>[2x]GPMVTGGGAAPPGTVTEPLPSVIVLSAGRKMAAAAAAASGPGCSSAAGAGAAGVSEWLVLRDGCMHCDADGLHSLSYHPALNAILAVTSRGTIKVIDGTSGATLQASALSAKPGGQVKCQYISAVDKVIFVDDYAVGCRKDLNGILLLDTALQTPVSKQDDVVQLELPVTEAQQLLSACLEKVDISSTEGYDLFITQLKDGLKNTSHETAANHKVAKWATVTFHLPHHVLKSIASAIVNELKKINQNVAALPVASSVMDRLSYLLPSARPELGVGPGRSVDRSLMYSEANRRETFTSWPHVGYRWAQPDPMAQAGFYHQPASSGDDRAMCFTCSVCLVCWEPTDEPWSEHERHSPNCPFVKGEHTQNVPLSVTLATSPAQFPCTDGTDRISCFGSGSCPHFLAAATKRGKICIWDVSKLMKVHLKFEINAYDPAIVQQLILSGDPSSGVDSRRPTLAWLEDSSSCSDIPKLEGDSDDLLEDSDSEEHSRSDSVTGHTSQKEAMEVSLDITALSILQQPEKLQWEIVANVLEDTVKDLEELGANPCLTNSKSEKTKEKHQEQHNIPFPCLLAGGLLTYKSPATSPISSNSHRSLDGLSRTQGESISEQGSTDNESCTNSELNSPLVRRTLPVLLLYSIKESDEKAGKIFSQMNNIMSKSLHDDGFTVPQIIEMELDSQEQLLLQDPPVTYIQQFADAAANLTSPDSEKWNSVFPKPGTLVQCLRLPKFAEEENLCIDSITPCADGIHLLVGLRTCPVESLSAINQVEALNNLNKLNSALCNRRKGELESNLAVVNGANISVIQHESPADVQTPLIIQPEQRNVSGGYLVLYKMNYATRIVTLEEEPIKIQHIKDPQDTITSLILLPPDILDNREDDCEEPIEDMQLTSKNGFEREKTSDISTLGHLVITTQGGYVKILDLSNFEILAKVEPPKKEGTEEQDTFVSVIYCSGTDRLCACTKGGELHFLQIGGTCDDIDEADILVDGSLSKGIEPSSEGSKPLSNPSSPGISGVDLLVDQPFTLEILTSLVELTRFETLTPRFSATVPPCWVEVQQEQQQRRHPQHLHQQHHGDAAQHTRTWKLQTDSNSWDEHVFELVLPKACMVGHVDFKFVLNSNITNIPQIQVTLLKNKAPGLGKVNALNIEVEQNGKPSLVDLNEEMQHMDVEESQCLRLCPFLEDHKEDILCGPVWLASGLDLSGHAGMLTLTSPKLVKGMAGGKYRSFLIHVKAVNERGTEEICNGGMRPVVRLPSLKHQSNKGYSLASLLAKVAAGKEKSSNVKNENTSGTRKSENLRGCDLLQEVSVTIRRFKKTSISKERVQRCAMLQFSEFHEKLLNTLCRKTDDGQITEHAQSLVLDTLCWLAGVHSNGPGSSKEGNENLLSKTRKFLSDIVRVCFFEAGRSIAHKCARFLALCISNGKCDPCQPAFGPVLLKALLDNMSFLPAATTGGSVYWYFVLLNYVKDEDLAGCSTACASLLTAVSRQLQDRLTPMEALLQTRYGLYSSPFDPVLFDLEMSGSSCKNVYNSSIGVQSDEIDLSDVLSGNGKVSSCTAAEGSFTSLTGLLEVEPLHFTCVSTSDGTRIERDDAMSSFGVTPAVGGLSSGTVGEASTALSSAAQVALQSLSHAMASAEQQLQVLQEKQQQLLKLQQQKAKLEAKLHQTTAAAAAAASAVGPVHNSVPSNPVAAPGFFIHPSDVIPPTPKTTPLFMTPPLTPPNEAVSVVINAELAQLFPGSVIDPPAVNLAAHNKNSNKSRMNPLGSGLALAISHASHFLQPPPHQSIIIERMHSGARRFVTLDFGRPILLTDVLIPTCGDLASLSIDIWTLGEEVDGRRLVVATDISTHSLILHDLIPPPVCRFMKITVIGRYGSTNARAKIPLGFYYGHTYILPWESELKLMHDPLKGEGESANQPEIDQHLAMMVALQEDIQCRYNLACHRLETLLQSIDLPPLNSANNAQYFLRKPDKAVEEDSRVFSAYQDCIQLQLQLNLAHNAVQRLKVALGASRKMLSETSNPEDLIQTSSTEQLRTIIRYLLDTLLSLLHASNGHSVPAVLQSTFHAQACEELFKHLCISGTPKIRLHTGLLLVQLCGGERWWGQFLSNVLQELYNSEQLLIFPQDRVFMLLSCIGQRSLSNSGVLESLLNLLDNLLSPLQPQLPMHRRTEGVLDIPMISWVVMLVSRLLDYVATVEDEAAAAKKPLNGNQWSFINNNLHTQSLNRSSKGSSSLDRLYSRKIRKQLVHHKQQLNLLKAKQKALVEQMEKEKIQSNKGSSYKLLVEQAKLKQATSKHFKDLIRLRRTAEWSRSNLDTEVTTAKESPEIEPLPFTLAHERCISVVQKLVLFLLSMDFTCHADLLLFVCKVLARIANATRPTIHLCEIVNEPQLERLLLLLVGTDFNRGDISWGGAWAQYSLTCMLQDILAGELLAPVAAEAMEEGTVGDDVGATAGDSDDSLQQSSVQLLETIDEPLTHDITGAPPLSSLEKDKEIDLELLQDLMEVDIDPLDIDLEKDPLAAKVFKPISSTWYDYWGADYGTYNYNPYIGGLGIPVAKPPANTEKNGSQTVSVSVSQALDARLEVGLEQQAELMLKMMSTLEADSILQALTNTSPTLSQSPTGTDDSLLGGLQAANQTSQLIIQLSSVPMLNVCFNKLFSMLQVHHVQLESLLQLWLTLSLNSSSTGNKENGADIFLYNANRIPVISLNQASITSFLTVLAWYPNTLLRTWCLVLHSLTLMTNMQLNSGSSSAIGTQESTAHLLVSDPNLIHVLVKFLSGTSPHGTNQHSPQVGPTATQAMQEFLTRLQVHLSSTCPQIFSEFLLKLIHILSTERGAFQTGQGPLDAQVKLLEFTLEQNFEVVSVSTISAVIESVTFLVHHYITCSDKVMSRSGSDSSVGARACFGGLFANLIRPGDAKAVCGEMTRDQLMFDLLKLVNILVQLPLSGNREYSARVSVTTNTTDSVSDEEKVSGGKDGNGSSTSVQGSPAYVADLVLANQQIMSQILSALGLCNSSAMAMIIGASGLHLTKHENFHGGLDAISVGDGLFTILTTLSKKASTVHMMLQPILTYMACGYMGRQGSLATCQLSEPLLWFILRVLDTSDALKAFHDMGGVQLICNNMVTSTRAIVNTARSMVSTIMKFLDSGPNKAVDSTLKTRILASEPDNAEGIHNFAPLGTITSSSPTAQPAEVLLQATPPHRRARSAAWSYIFLPEEAWCDLTIHLPAAVLLKEIHIQPHLASLATCPSSVSVEVSADGVNMLPLSTPVVTSGLTYIKIQLVKAEVASAVCLRLHRPRDASTLGLSQIKLLGLTAFGTTSSATVNNPFLPSEDQVSKTSIGWLRLLHHCLTHISDLEGMMASAAAPTANLLQTCAALLMSPYCGMHSPNIEVVLVKIGLQSTRIGLKLIDILLRNCAASGSDPTDLNSPLLFGRLNGLSSDSTIDILYQLGTTQDPGTKDRIQALLKWVSDSARVAAMKRSGRMNYMCPNSSTVEYGLLMPSPSHLHCVAAILWHSYELLVEYDLPALLDQELFELLFNWSMSLPCNMVLKKAVDSLLCSMCHVHPNYFSLLMGWMGITPPPVQCHHRLSMTDDSKKQDLSSSLTDDSKNAQAPLALTESHLATLASSSQSPEAIKQLLDSGLPSLLVRSLASFCFSHISSSESIAQSIDISQDKLRRHHVPQQCNKMPITADLVAPILRFLTEVGNSHIM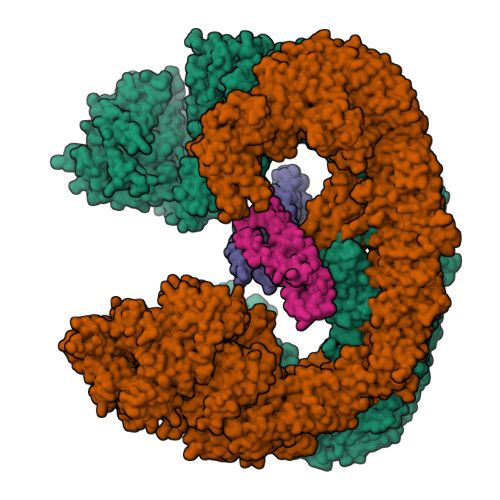KDWLGGSEVNPLWTALLFLLCHSGSTSGSHNLGAQQTSARSASLSSAATTGLTTQQRTAIENATVAFFLQCISCHPNNQKLMAQVLCELFQTSPQRGNLPTSGNISGFIRRLFLQLMLEDEKVTMFLQSPCPLYKGRINATSHVIQHPMYGAGHKFRTLHLPVSTTLSDVLDRVSDTPSITAKLISEQKDDKEKKNHEEKEKVKAENGFQDNYSVVVASGLKSQSKRAVSATPPRPPSRRGRTIPDKIGSTSGAEAANKIITVPVFHLFHKLLAGQPLPAEMTLAQLLTLLYDRKLPQGYRSIDLTVKLGSRVITDPSLSKTDSYKRLHPEKDHGDLLASCPEDEALTPGDECMDGILDESLLETCPIQSPLQVFAGMGGLALIAERLPMLYPEVIQQVSAPVVTSTTQEKPKDSDQFEWVTIEQSGELVYEAPETVAAEPPPIKSAVQTMSPIPAHSLAAFGLFLRLPGYAEVLLKERKHAQCLLRLVLGVTDDGEGSHILQSPSANVLPTLPFHVLRSLFSTTPLTTDDGVLLRRMALEIGALHLILVCLSALSHHSPRVPNSSVNQTEPQVSSSHNPTSTEEQQLYWAKGTGFGTGSTASGWDVEQALTKQRLEEEHVTCLLQVLASYINPVSSAVNGEAQSSHETRGQNSNALPSVLLELLSQSCLIPAMSSYLRNDSVLDMARHVPLYRALLELLRAIASCAAMVPLLLPLSTENGEEEEEQSECQTSVGTLLAKMKTCVDTYTNRLRSKRENVKTGVKPDASDQEPEGLTLLVPDIQKTAEIVYAATTSLRQANQEKKLGEYSKKAAMKPKPLSVLKSLEEKYVAVMKKLQFDTFEMVSEDEDGKLGFKVNYHYMSQVKNANDANSAARARRLAQEAVTLSTSLPLSSSSSVFVRCDEERLDIMKVLITGPADTPYANGCFEFDVYFPQDYPSSPPLVNLETTGGHSVRFNPNLYNDGKVCLSILNTWHGRPEEKWNPQTSSFLQVLVSVQSLILVAEPYFNEPGYERSRGTPSGTQSSREYDGNIRQATVKWAMLEQIRNPSPCFKEVIHKHFYLKRVEIMAQCEEWIADIQQYSSDKRVGRTMSHHAAALKRHTAQLREELLKLPCPEGLDPDTDDAPEVCRATTGAEETLMHDQVKPSSSKELPSDFQL;>AVPIAQKSEPHSLSSEALMRRAVSLVTDSTSTFLSQTTYALIEAITEYTKAVYTLTSLYRQYTSLLGKMNSEEEDEVWQVIIGARAEMTSKHQEYLKLETTWMTAVGLSEMAAEAAYQTGADQASITARNHIQLVKLQVEEVHQLSRKAETKLAEAQIEELRQKTQEEGEERAESEQEAYLRED[2x]>MTKHYDYIAIGGGSGGIASINRAAMYGQKCALIEAKELGGTCVNVGCVPKKVMWHAAQIREAIHMYGPDYGFDTTINKFNWETLIASRTAYIDRIHTSYENVLGKNNVDVIKGFARFVDAKTLEVNGETITADHILIATGGRPSHPDIPGVEYGIDSDGFFALPALPERVAVVGAGYIGVELGGVINGLGAKTHLFEMFDAPLPSFDPMISETLVEVMNAEGPQLHTNAIPKAVVKNTDGSLTLELEDGRSETVDCLIWAIGREPANDNINLEAAGVKTNEKGYIVVDKYQNTNIEGIYAVGDNTGAVELTPVAVAAGRRLSERLFNNKPDEHLDYSNIPTVVFSHPPIGTVGLTEPQAR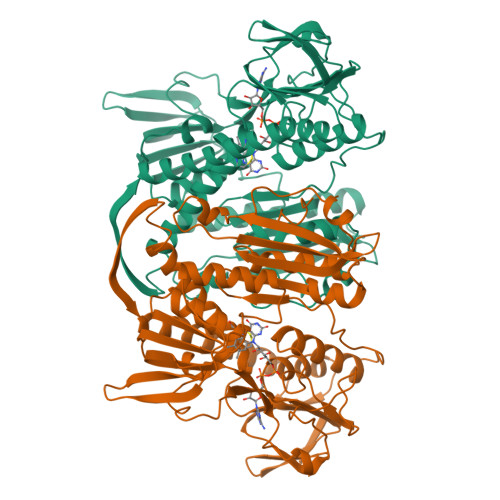EQYGDDQVKVYKSSFTAMYTAVTTHRQPCRMKLVCVGSEEKIVGIHGIGFGMDEMLQGFAVALKMGATKKDFDNTVAIHPTAAEEFVTMR[2x]> MGSDYKDHDGDYKDHDIDYKDDDDKGSGSLEVLFQGPMDPIINGNSANVYLTDSYLKGVISFSECNALGSYIFNGPYLKNDYTNLISRQNPLIEHMNLKKLNITQSLISKYHKGEIKLEEPTYFQSLLMTYKSMTSSEQIATTNLLKKIIRRAIEISDVKVYAILNKLGLKEKDKIKSNNGQDEDNSVITTIIKDDILSAVKDNQSHLKADKNHSTKQKDTIKTTLLKKLMCSMQHPPSWLIHWFNLYTKLNNILTQYRSNEVKNHGFTLIDNQTLSGFQFILNQYGCIVYHKELKRITVTTYNQFLTWKDISLSRLNVCLITWISNCLNTLNKSLGLRCGFNNVILTQLFLYGDCILKLFHNEGFYIIKEVEGFIMSLILNITEEDQFRKRFYNSMLNNITDAANKAQKNLLSRVCHTLLDKTVSDNIINGRWIILLSKFLKLIKLAGDNNLNNLSELYFLFRIFGHPMVDERQAMDAVKINCNETKFYLLSSLSMLRGAFIYRIIKGFVNNYNRWPTLRNAIVLPLRWLTYYKLNTYPSLLELTERDLIVLSGLRFYREFRLPKKVDLEMIINDKAISPPKNLIWTSFPRNYMPSHIQNYIEHEKLKFSESDKSRRVLEYYLRDNKFNECDLYNCVVNQSYLNNPNHVVSLTGKERELSVGRMFAMQPGMFRQVQILAEKMIAENILQFFPESLTRYGDLELQKILELKAGISNKSNRYNDNYNNYISKCSIITDLSKFNQAFRYETSCICSDVLDELHGVQSLFSWLHLTIPHVTIICTYRHAPPYIGDHIVDLNNVDEQSGLYRYHMGGIEGWCQKLWTIEAISLLDLISLKGKFSITALINGDNQSIDISKPIRLMEGQTHAQADYLLALNSLKLLYKEYAGIGHKLKGTETYISRDMQFMSKTIQHNGVYYPASIKKVLRVGPWINTILDDFKVSLESIGSLTQELEYRGESLLCSLIFRNVWLYNQ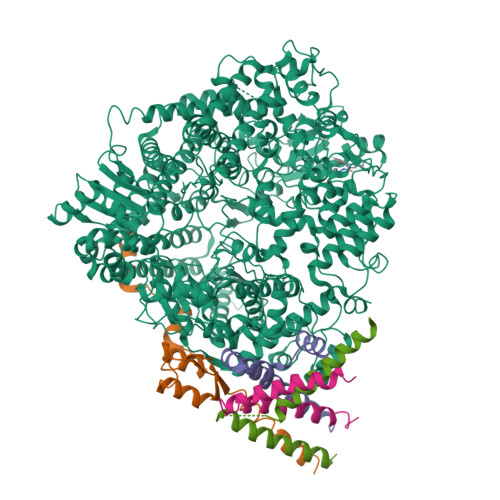IALQLKNHALCNNKLYLDILKVLKHLKTFFNLDNIDTALTLYMNLPMLFGGGDPNLLYRSFYRRTPDFLTEAIVHSVFILSYYTNHDLKDKLQDLSDDRLNKFLTCIITFDKNPNAEFVTLMRDPQALGSERQAKITSEINRLAVTEVLSTAPNKIFSKSAQHYTTTEIDLNDIMQNIEPTYPHGLRVVYESLPFYKAEKIVNLISGTKSITNILEKTSAIDLTDIDRATEMMRKNITLLIRILPLDCNRDKREILSMENLSITELSKYVRERSWSLSNIVGVTSPSIMYTMDIKYTTSTISSGIIIEKYNVNSLTRGERGPTKPWVGSSTQEKKTMPVYNRQVLTKKQRDQIDLLAKLDWVYASIDNKDEFMEELSIGTLGLTYEKAKKLFPQYLSVNYLHRLTVSSRPCEFPASIPAYRTTNYHFDTSPINRILTEKYGDEDIDIVFQNCISFGLSLMSVVEQFTNVCPNRIILIPKLNEIHLMKPPIFTGDVDIHKLKQVIQKQHMFLPDKISLTQYVELF;>[4x]MEKFAPEFHGEDANNRATKFLESIKGKFTSPKDPKKKDSIISVNSIDIEVTKESPITSNSTIINPTNETDDTAGNKPNYQRKPLVSFKEDPTPSDNPFSKLYKETIETFDNNEEESSYSYEEINDQTNDNITARLDRIDEKLSEILGMLHTLVVASAGPTSARDGIRDAMIGLREEMIEKIRTEALMTNDRLEAMARLRNEESEKMAKDTSDEVSLNPTSEKLNNLLEGNDSDNDLSLEDFKGENKYFQGHHHHHH> TRDQNGTWEMESNENFEGWMKAL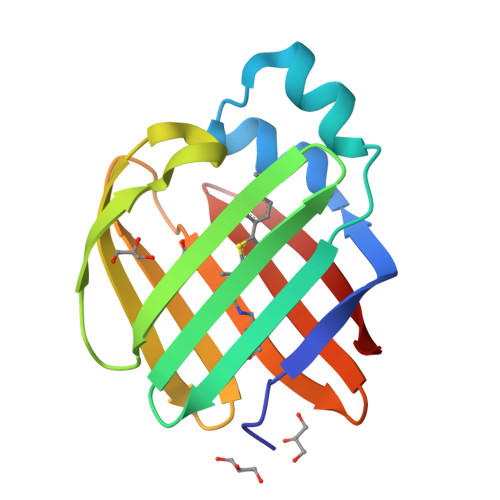DIDFATRKIWVRLTQTLVIDQDGDNFKVKSTSTFWNYDVDFTVGVEFDEYTKSLDNRHVKALVTWEGDVLVCVQKGEKENRGWKKWIEGDKLYEELTCGDQVCRQVFKKK> DVSTSELDQFEFWVQYAAASYYEADYTAQVGDKLSCSKGNCPEVEATGATVSYDFSDSTITDTAGYIAVDHTNSAVVLAFRGSYSVRNWVADATFVHTNPGLCDGCLAELGFWSSWKLVRDDIIKELKEVVAQNPNYEL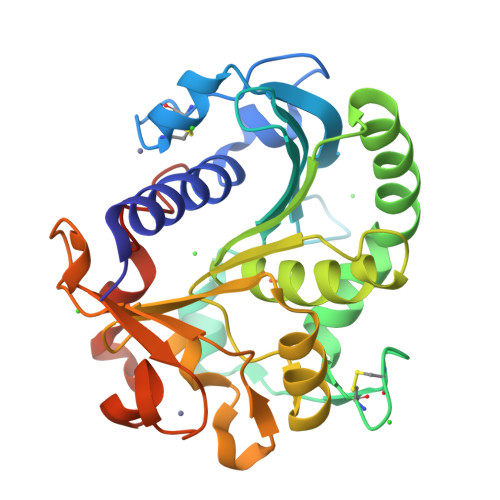VVVGHSLGAAVATLAATDLRGKGYPSAKLYAYASPRVGNAALAKYITAQGNNFRFTHTNDPVPKLPLLSMGYVHVSPEYWITSPNQATVSTSDIKVIDGDVSFDGNTGTGLPLLTDFEAHIWYFVQVDAGKGPGLPFKRV> MGSDKIHHHHHHENLYFQGMRNMQEKGVSEKEILEELKKYRSLDLKYEDGNIFGSMCSNVLPITRKIVDIFLETNLGDPGLFKGTKLLEEKAVALLGSLLNNKDAYGHIVSGGTEANLMALRCIKNIWREKRRKGLSKNEHPKIIVPITAHFSFEKGREMMDLEYIYAPIKEDYTIDEKFVKDAVEDYDVDG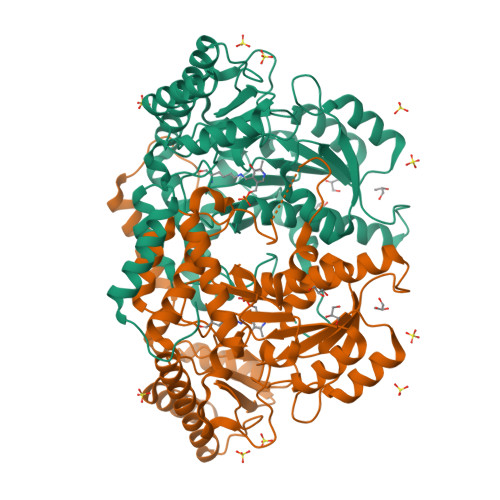IIGIAGTTELGTIDNIEELSKIAKENNIYIHVDAAFGGLVIPFLDDKYKKKGVNYKFDFSLGVDSITIDPHKMGHCPIPSGGILFKDIGYKRYLDVDAPYLTETRQATILGTRVGFGGACTYAVLRYLGREGQRKIVNECMENTLYLYKKLKENNFKPVIEPILNIVAIEDEDYKEVCKKLRDRGIYVSVCNCVKALRIVVMPHIKREHIDNFIEILNSIKRD> GSMAAAGNKSINAKLVLLGDVGAGKSS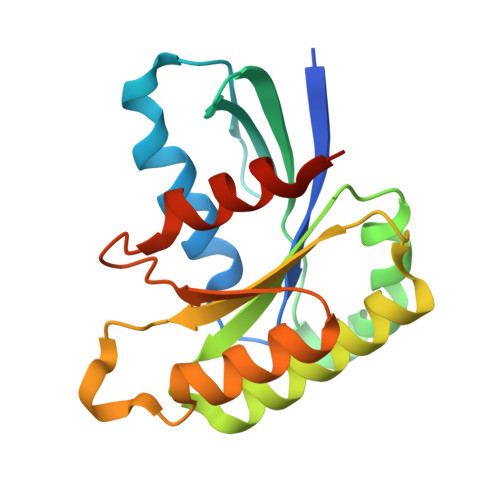LVLRFVKDQFVEFQESTIGAAFFSQTLAVNDATVKFEIWDTAGQERYHSLAPMYYRGAAAAIIVFDVTNQASFERAKKWVQELQAQGNPNMVMALAGNKSDLLDARKVTAEDAQTYAQENGLFFMETSAKTATNVKEIFYEIARRLPRVQPTEN>PSVYDAAAQLTADVKKDLRDSWKVIGSDKKGNGVALMTTLFADNQETIGYFKRLGDVSQGMANDKLRGHSITLMY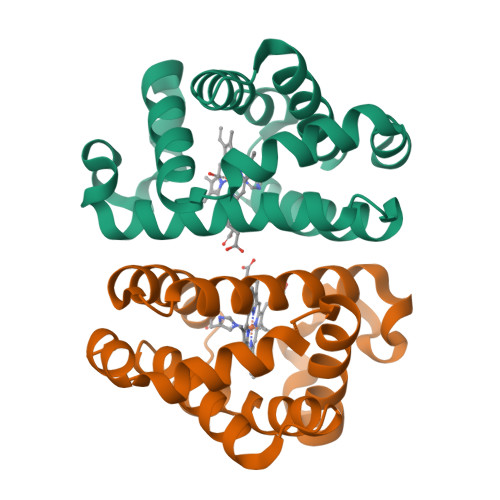ALQNFIDQLDNPDDLVCVVEKFAVAHITRKISAAEFGKINGPIKKVLASKNFGDKYANAWAKLVAVVQAAL[2x]The sulfonamides (sulfas) are the oldest class of antibacterial drugs and inhibit the bacterial dihydropteroate synthase (DHPS, encoded by folP), through chemical mimicry of its co-substrate p-aminobenzoic acid (pABA). Resistance to sulfa drugs is mediated either by mutations in folP or acquisition of sul genes, which code for sulfa-insensitive, divergent DHPS enzymes. DHPS catalyzes the condensation of para-aminobenzoic acid (pABA) and 6-hydroxymethyl-7,8-dihydropterin pyrophosphate (DHPP), producing 7,8-dihydropteroic acid (7,8-DHP); this compound is further transformed, ultimately leading to tetrahydrofolate, an essential precursor for DNA and RNA synthesis. All three Sul enzymes adopted the (ɑ/β)8 TIM barrel fold also shared by DHPS.

The Sul3·DHP+·Mg2+·pABA complex structure also featured a well-defined active site. This Sul complex structure contained electron density corresponding to DHP+21, pABA, Mg2+ and PPi. Multiple electron density features verify this trapped molecule is DHP+, including a clear break between its C9 position and the p-amino group of pABA, and a ring pucker around atoms C6, C7 and N8 consistent with saturation at the C7 position. The position of DHP+ in the Sul3·DHP+·pABA·Mg2+·PPi complex superimposed with its position in the YpDHPS transition state complex structure 21 and the pterin ring in the Sul2·7,8-DHP·Mg2+·PPi complex. All the protein-ligand interactions observed in the Sul2·7,8-DHP·Mg2+·PPi complex were consistent with those observed in the Sul3·DHP+·pABA·Mg2+·PPi complex, including the hydrophobic interaction between pABA and Phe177. Furthermore, the conserved Phe residue belonging to this helix (Phe178 in Sul1, Phe179 in Sul2, Phe177 in Sul3) and providing an additional hydrogen bond to pABA through its backbone amide nitrogen is lacking in DHPS enzymes. The sidechain of this residue in the Sul enzyme structures was localized near the carboxylic acid group of pABA and occupied a spatial location that would clash with the sulfonamide group and its N-acylation (i.e., the azole group of SMX) as revealed in the YpDHPS·DHPP·SMX complex structure.

> GMSKIFGIVNITTDSFSDGGLYLDTDKAIEHALHLVEDGADVIDLGAASSNPDTTEVGVVEEIKRLKPVIKALKEKGISISVDTFKPEVQSFCIEQKVDFINDIQGFPYPEIYSGLAKSDCKLVLMHSVQRIGAATKVETNPAAVFTSMMEFFKERIAALVEAGVKRERIILDPGMGFFLGSNPETSILVLKRFPEIQEAFNLQVMIAVSRKSFLGKITGTDVKSRLAPTLAAEMYAYKKGADYLRTHDVKSLSDALKISKALG>[6x]MGESKRTEKTRVLVVGATGYIGKRIVRACLAEGHETYVLQRPEIGLEIEKVQLFLSFKKLGARIVEGSFSDHQSLVSAVKLVDVVV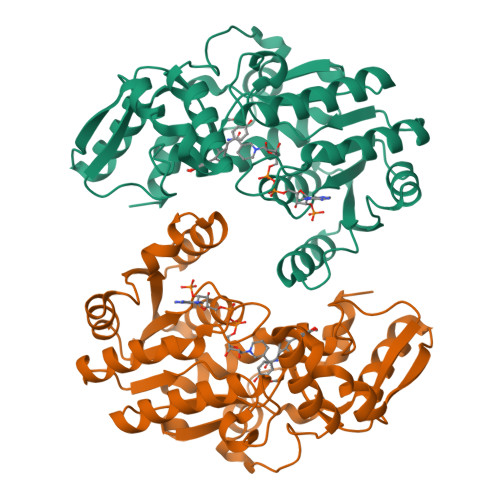SAMSGVHFRSHNILVQLKLVEAIKEAGNVKRFLPSEFGMDPPRMGHALPPGRETFDQKMEVRQAIEAAGIPYTYVVGACFAAYFAGNLSQMVTLLPPKEKVNIYGDGNVKVVFADEDDIAKYTAKTLNDPRTLNKTVNIRPPDNVLTQLELVQIWEKLTGKELEKTNIAAQDFLANIEQMEIPHQAGIGHFYHIFYEGCLTDHEVGEDEEASSLYPDVKYKRMDDYLRMFL>[2x]QGTNVNDKVHFTNIDIAIDKGHVNKTTGNTEFWATSSDVLKLK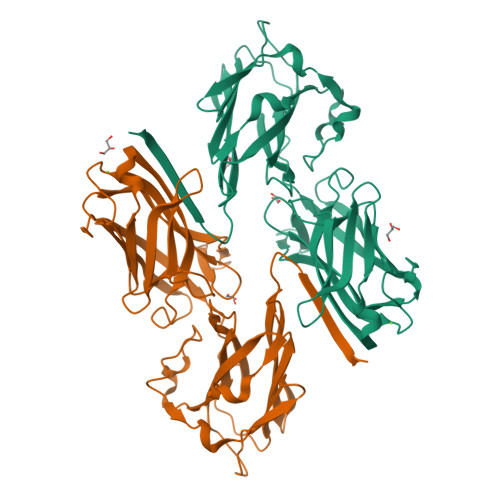ANYTIDDSVKEGDTFTFKYGQYFRPGSVRLPSQTQNLYNAQGNIIAKGIYDSKTNTTTYTFTNYVDQYTNVSGSFEQVAFAKRENATTDKTAYKMEVTLGNDTYSKDVIVDYGNQKGQQLISSTNYINNEDLSRNMTVYVNQHKKTYTKETFVTNLTGYKFNPDAKNFKIYEVTDQNQFVDSFTPDTSKLKDVTGQFDVIYSNDNKTATVDLLNGQSSSDKQYIIQQVAYPDNSSTDNGKIDYTLETQNGKSSWSNSYSNVNGSSTANGDQK>[2x]MSLAKPIEAHTVSPVNP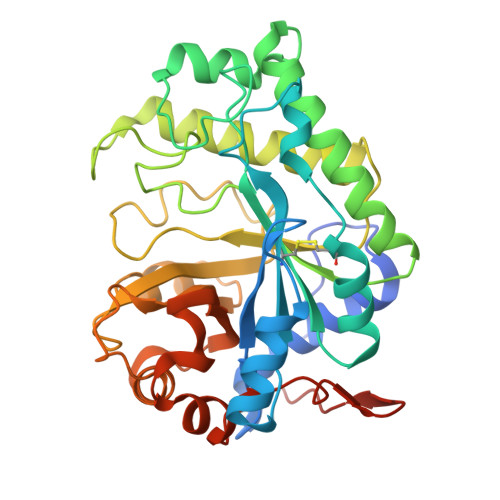NAQQTTKTVMNWLAHLPNRTENRVLSGAFGGYSHDTFSMAEADRIRSATGQSPAIYGCDYARGWLETANIEDSIDVSCNGDLMSYWKNGGIPQISLHLANPAFQSGHFKTPITNDQYKKILDSSTVEGKRLNAMLSKIADGLQELENQGVPVLFRPLHEMNGEWFWWGLTSYNQKDNERISLYKQLYKKIYHYMTDTRGLDHLIWVYSPDANRDFKTDFYPGASYVDIVGLDAYFQDAYSINGYDQLTALNKPFAFTEVGPQTANGSFDYSLFINAIKQKYPKTIYFLAWNDEWSAAVNKGASALYHDSWTLNKGEIWNGDSLTPIVEEGHHHHHH>GPRMAFTNYSSLNRAQLTFEYLHTNSTTHEFLFGALAELVDNARDADATRIDIYAERREDLRGGFMLCFLDDGAGMDPSDAASVIQFGKLAKRTPESTQIGQYGNGLKSGSMRIGKDFILFTKKEDTMTCLFLSRTFHEEEGIDEVIVPLPTWNARTREPVTDNVEKFAIETELIYKYSPFRTEEEVMTQFMKIPGDSGTLVIIFNLKLMDNGEPELDIISNPRDIQMAETSPEGTKPERRSFRAYAAVLYIDPRMRIFIHGHKVQTKRLSCCLYKPRMYKYTSSRFKTRAEQEVKKAEHVARIAEEKAREAESKARTLEVRLGGDLTRDSRVMLRQVQNRAITLRREADVKKRIKEAKQRALKEPKELNFVFGVNIEHRDLDGMFIYNCSRLIKMYEKVGPQLEGGMACGGVVGVVDVPYLVLEPTHNKQDFADAKEYRHLLRAMGEHLAQYWKDIAIAQRGIIKFWDEFGYLSANWNQPPSSELRYKRRRAMEIPTTIQCDLCLKWRTLPFQLSSVEKDYPDTWVCSMNPDPEQDRCEASEQKQKVPLGTFRKDMKTQEEKQKQLTEKIRQQQEKLEALQKTTPIRSQADLKKLPLEVTTRPST[2x]

Microrchidia CW-type zinc finger proteins (MORCs) are a family of transcriptional regulators conserved in eukaryotes. We recently showed that human MORC2 is necessary, in conjunction with the human silencing hub (HUSH), for silencing of transgenes integrated at chromatin loci with histone H3 trimethylated at lysine 9 H3K9me3. MORC2 is a 1032-amino acid protein predicted to contain several functional domains including an N-terminal GHKL-type ATPase module with a coiled-coil insertion (CC1). Here we report the biochemical and cellular activities of MORC2 variants, alongside structures of wild-type and neuropathic variant forms of a MORC2 fragment comprising the GHKL-type ATPase module and CW domain.

T424R MORC2 was co-crystallized with AMPPNP using the same protocol as for wild-type MORC2, but since S87L was dimeric and nucleotide-bound upon purification from insect cells, we determined its structure bound to ATP. The ATP molecules bound to S87L MORC2 were found in a nearly identical conformation to AMPPNP in the wild-type and T424R structures, confirming that AMPPNP is a reasonable mimic of the natural nucleotide substrate in this case. Ser87 is in the lid that covers bound ATP. Its sidechain hydroxyl forms a hydrogen bond with the β-phosphate of AMPPNP in the wild-type structure. In the S87L mutant, we found that the lid is partially missing in one protomer and has a completely different conformation in the other. In the latter protomer, the lid forms additional contacts across the dimer interface in the S87L mutant. Leu87 itself forms apolar contacts with Asp141 from the other protomer, but more importantly, Arg90 forms a tight salt bridge with Glu17 across protomers. The increased number of dimer contacts in the S87L mutant is reflected in an increased buried surface area at the dimer interface (3016 Å2 buried per protomer versus 2778 Å2 in wild-type). These observations provide a plausible structural basis for the observation that S87L forms more stable ATP-bound dimers than wild-type, which in turn affects its cellular function. S87L (which has reduced ATPase activity in vitro) also matched or outperformed wild-type MORC2 at each time point measured.>STLEVRSQATQDLSEYYNRPYFDLRNLSGYREGNTVTFINHYQQTDVKLEGKDKDKIKDGNNENLDVFVVREGSGRQADNNSIGGITKTNRTQHIDTVQNVNLLVSKSTGQHTTSVTSTNYSIYKEEISLKELDFKLRKHLIDKHDLYKTEPKDSKIRVTMKNGDFYTFELNKKLQTHRMGDVIDGRNI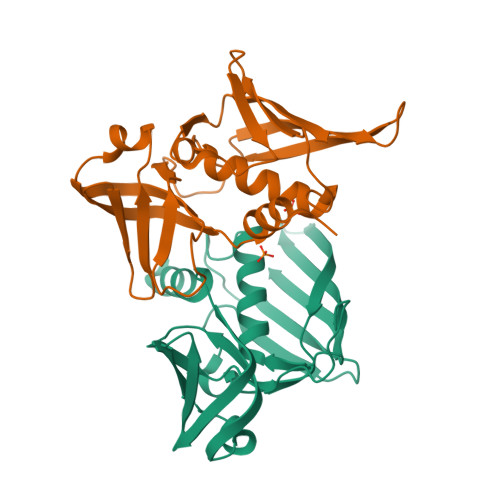EKIEVNL[4x]>[2x]GET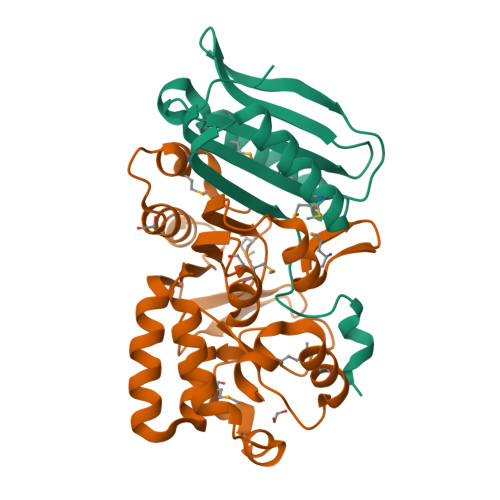PEPRTTRTILVYMMANNSLNSFASKNIESMIEGATSKNLNGGNLIVYYAPAGSPPELLRIKEENGVVKKIHLKDYEKQNSADPDVMRSVIGEVVSQYPADSYGLVLWSHGTAWLPSDYQNKLK;>AFGQDGNNWMEIDDLAKGLPDDLFDFILFDACYMASVECTYELRNKAEYILASPTETMADGWPYEEMMPQLFATDLQLEKVGETFYNHYLNNTYPYATVSLTKTSELDNLKSAIHDILADKTESDIYSLDPKNMQRLEYLYRSPGMLYDFNDYIKQLATAEQYDRFISCLDKAVVYKAHTPKSYYAAIGNALPIKSYCGLTIFVPQESLPKMLEWYKQRVGWYKAVYE[2x]>[4x]GDIVSEKKPA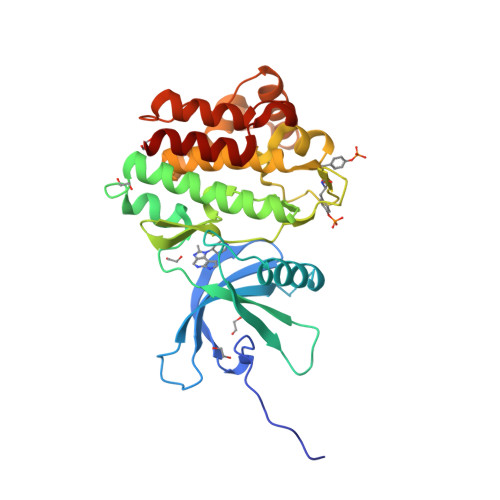TEVDPTHFEKRFLKRIRDLGEGHFGKVELCRYDPEGDNTGEQVAVKSLKPESGGNHIADLKKEIEILRNLYHENIVKYKGICTEDGGNGIKLIMEFLPSGSLKEYLPKNKNKINLKQQLKYAVQICKGMDYLGSRQYVHRDLAARNVLVESEHQVKIGDFGLTKAIETDKEYYTVKDDRDSPVFWYAPECLMQSKFYIASDVWSFGVTLHELLTYCDSDSSPMALFLKMIGPTHGQMTVTRLVNTLKEGKRLPCPPNCPDEVYQLMRKCWEFQPSNRTSFQNLIEGFEALLK>[2x]AAPPPINKLALFPDKSAWCEAK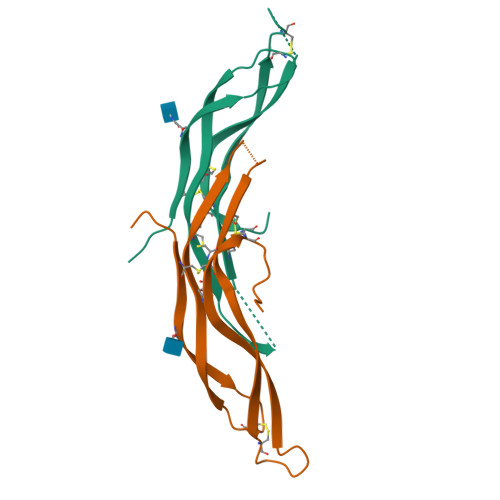NITQIVGHSGCEAKSIQNRACLGQCFSYSVPNTFPQSTESLVHCDSCMPAQSMWEIVTLECPGHEEVPRVDKLVEKILHCSCQACGKEPSHEGL>[4x]MTARTERGRALAFVWLMVEGAQVAAGGVAGYVRNLLDEQD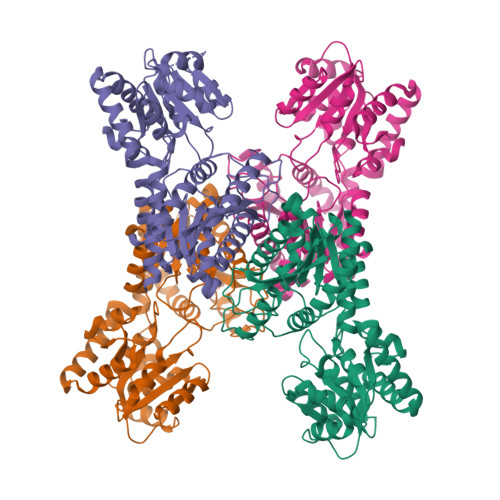ALRDHLAERGWSVEFVLGEPFYDPGAPGYDEERWRRVREHLAARGGRAVRLVSDSDGLDGWGEERFFHALSATGAQLVLDTAERCDAVVAVSGTSAFARVPGMVQRQGGELAAKVLHVHTFGLATHDTAHVPSPAEIAADGDVAFWTRQSDRVSVGYISRYTAELYARTYAIPAAALLPNRSAIPRHAPRFGVLTEERINERIAGLGLPAEGEFVVMWGRNSAPGLDKGYHLLLEAARDLPGVVPVIATRRPDPGLRRLADRYAVPAVLLDDQPFTHLSALLQSPRTLAAAFLGEAEPGAVSPMEAMWVARESGALVIAADTGNLPEVVDDGAAGIVTRRTAADVADAVRRVRKLTADERRRMRAAAAARVRARFDFAANVRELADAAVDRLAEVSKLAAALEHHHHHHHH>[2x]DVSGSLRIAIPVSFSQELIANLCSGFMRLYPNVELDVQFTDNDIGLVGEGYDIAIKYGPLQSSDLVARLLFERQPILVASPGYLKTRGTPATPKELSDHSGILLGTSRSAPIWPLGKGTRKTMVSFQRKVRVNSPIMVKQLALDDFGIAMLSNSACKTELANGQLVPILQEWPMEPFKVYGVYSSRRQLATNISAFLDFFVKRFSSQESLQSLM

Here, we describe the discovery of a LysR type transcriptional regulator (LTTR), AccR (for ACCase regulator) in S. oneidensis, which directly and specifically activates transcription of the accS gene as a canonical LTTR. Like other LTTRs, AccR is predicted to form a N-terminal winged helix-turn-helix (wHTH) DNA-binding domain (DBD) and a C-terminal EBD (also called regulatory domain, RD) that are connected by a linker made of an extended helix and a flexible hinge. We showed that AccR interacts with the accS promoter in vivo in response to changes in acetyl-CoA levels and in vitro. Multiple lines of evidence indicate that acetyl-CoA is one of the effectors.

Despite numerous trials, we were not able to obtain any crystal hits for the full-length AccR. EBD crystals were rod-shaped, belonging to the space group C2. An EBD dimer was found in each asymmetric unit, with the two subunits arranged in an antiparallel manner. The final structural model of AccR EBD contains residues 89–302 for subunit A and residues 90–300 for the subunit B, except for residues 132–136 and 206–207 in two surface loops of the subunit B that are structurally disordered. Superimposition of the two EBD subunits in a dimer gave an overall r.m.s.d. of 0.25 Å for 204 common Cα atoms, suggesting nearly identical conformation. In the AccR EBD dimer, ∼3200 Å2 of surface area is buried at the dimer interface, which is mostly mediated by α5, β4 with α7 and β10 from the adjacent subunit, suggesting stable molecular interactions. Structural comparison indicates that AccR EBD has a large, ‘primary’ funnel-shaped ligand binding pocket within a monomer. This funnel-shaped pocket, which runs through the entire molecule, is 25 Å by 20 Å wide near its opening, with most of the surface being neutral to positively charged. In addition, another ‘secondary’ pocket is found at the regulatory domain dimerization interface and contains S103 and E105 from both chains of the dimer. However, this secondary pocket found in AccR may not interact with acetyl-CoA because it is a negatively charged cavity as seen by the surface charge representation, and acetyl-CoA is also negatively charged.>GPDEKTVPNFKSPDPDYPWYGYDSYRGIFARYHNLKVNLKGSKEYQAYCFNLTKYFPRPTYSTTNNFYKKIDGSGSAFKSYAANPRVLDENLDKLEKNILNVIYNGYKSNANGFMNGIEDLNAILVTQNAIWYYSDSAPLNDVNKMWEREVRNGEISESQVTLMREALKKLIDPNLEATAANKIPSGYRLNIFKSENEDYQNLLSAEYV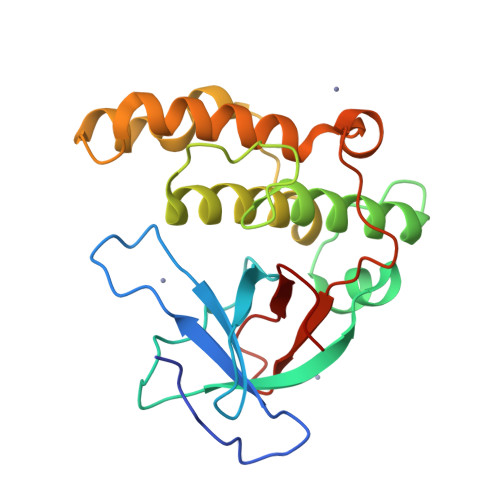P[2x]>[2x]MAFKLPNLPYAYDALEPYIDQRTMEFHHDKHHNTYVTKLNATVEGTELEHQSLADMIANLDKVPEAMRMSVRNNGGGHFNHSLFWEILSPNSEEKGGVIDDIKAQWGTLDEFKNEFANKATTLFGSGWTWLVVNDGKLEIVTTPNQDNPLTEGKTPILGLDVWEHAYYLKYQNKRPDYMTAFWNIVNWKKVDELYQAAK

SODs detoxify superoxide, a reactive oxygen radical produced by aerobic metabolism and by the mammalian immune system in response to infection. We recently established that a Mn/Fe SOD from the bacterium Staphylococcus aureus exhibits equal activity with either manganese or iron. In addition to the camSOD (SodM), S. aureus also possesses a second, manganese-dependent SOD (SodA). All members of the Mn/Fe SOD family are related in sequence, exhibit identical protein folds, and coordinate their metal ion using identical ligands, making it unclear why some enzymes absolutely require manganese for catalysis (MnSOD), while others require iron (FeSOD), and still others show metal cofactor flexibility (camSOD).

Remarkably, the chemical differences between the sidechains of these residues are minor, with Gly (MnSOD) and Leu (camSOD) at position 159, and Leu (MnSOD) and Phe (camSOD) at position 160. Conversely, the camSOD double mutant (Leu159Gly-Phe160Leu) had greater activity with manganese and reduced activity with iron relative to the wild type or the single mutant (camSOD Leu159Gly). This shift in camSOD metal preference resulted in a highly manganese-specific enzyme (CR = 0.016). Cumulatively, these results demonstrate that just two mutations in the secondary coordination sphere largely interconvert the metal specificity of camSOD and MnSOD. The camSOD triple mutant (Ile19Phe-Leu159Gly-Phe160Leu) had increased activity with both metals relative to the double mutant (camSOD Leu159Gly-Phe160Leu). These studies demonstrate that positions 159 and 160 are important in regulating the reactivity of the metal cofactor. Strikingly, mutations at these positions produced profound effects on metal specificity, yet did so with essentially no changes to the protein backbone structure, at least within the resolution of the crystal structures. Altogether, the spectroscopic data indicate that the two wild-type S. aureus SODs and the two double mutants differ in their manganese redox properties. The auto-oxidation data and dithionite reduction data both suggest that the two wild-type SODs have different reduction potentials. These differences are inverted in the double mutants in both assays, which correlates with the inversion of manganese-dependent activity in these variants. The double mutation in MnSOD resulted in an altered electronic structure and re-tuning of the manganese reduction potential to more closely match that of camSOD and more catalytically active with iron, whereas the camSOD mutations altered reduction potential to make it more similar to MnSOD and more catalytically active with manganese.Members of the SET and MYND domain containing (SmyD) family of proteins possess histone lysine methyltransferase capacity and have been shown to be involved in the transcriptional control of cell differentiation and cell proliferation. Interest in SmyD2 has grown significantly because of recent reports indicating that SmyD2 repress transcriptional p53 activity by lysine methylation (Lys370), exerting an oncogenic and drug resistance action through inhibition of p53-mediated cell death pathways. The N-terminal lobe (residues 3–279) is composed of four domains: the catalytic SET domain, located in the middle of this lobe, is surrounded by the zinc finger MYND, insertion SET-I, and post-SET domains. Immediately C-terminal to the post-SET domain, the polypeptide forms a large domain of about 150 residues that constitutes the C-terminal lobe (residues 280–432).

We have determined two complex structures of SmyD2 bound either to the cofactor product AdoHcy or to a potent methyltransferase inhibitor sinefungin. The two structures are remarkably similar to each other in terms of cofactor binding. Significantly, the two SmyD2 structures in complex with the cofactor analogs sinefungin and AdoHcy differ dramatically in the conformation of the CTD. Despite that the structures of SmyD2–SFG and SmyD2–AdoHcy are highly superimposable with RMSD of 0.36 Å over 400 residues, close examination reveals that the first two helices of the CTD (αH and αI) adopt different conformations. In agreement with the conformational changes, the flexible nature of the αH and αI helices is also indicated by their higher than average isotropic temperature factors of 41.9 Å2 for SmyD2–AdoHcy and 39.5 Å2 for SmyD2–SFG. There are, however, some differences caused by the CTD motion in the interaction networks between the CTD and post-SET domain, including a new hydrogen bond between the side chains of Arg299 and Glu248 and the potential salt-bridge interactions between Arg306 and Asp256 in SmyD2–AdoHcy. The overall crystal packing is effectively identical in the SmyD2–AdoHcy and SmyD2–sinefungin complexes, except at the packing interfaces that involve αH and αI. The different orientations of these two helices are stabilized by the differences in crystal packing contacts that contain spatially close but distinct sets of residues. Based on these analyses, we propose a model of SmyD2 activation by Hsp90, in which the Hsp90 MEEVD motif could compete with the β8–β9 hairpin for binding to the SmyD2 CTD, displacing the CTD from the substrate binding site and causing a conformational change in the CTD. This model is in agreement with the conformational flexibility of the CTD as revealed by the structural differences between SmyD2–AdoHcy and SmyD2–SFG.

> MRAEARGGLERFCSAGKGRGLRALRPFHVGDLLFSCPAYACVLTVGERGHHCECCFARKEGLSKCGRCKQAFYCDVECQKEDWPLHKLECSSMVVLGENWNPSETVRLTARILAKQKIHPERTPSEKLLAVREFESHLDKLDNEKKDLIQSDIAALHQFYSKYLEFPDHSSLVVLFAQVNCNGFTIEDEELSHLGSAIFPDVALMNHSCCPNVIVTYKGTLAEVRAVQEIHPGDEVFTSYIDLLYPTEDRNDRLRDSYFFTCECRECTTKDKDKAKVEVRKLSSPPQAEAIRDMVRYARNVIEEFRRAKHYKSPSELLEICELSQEKMSSVFEDSNVYMLHMMYQAMGVCLYMQDWEGALKYGQKIIKPYSKHYPVYSLNVASMWLKLGRLYMGLENKAAGEKALKKAIAIMEVAHGKDHPYISEIKQEIESH> MTVGTLVASVLPATVFE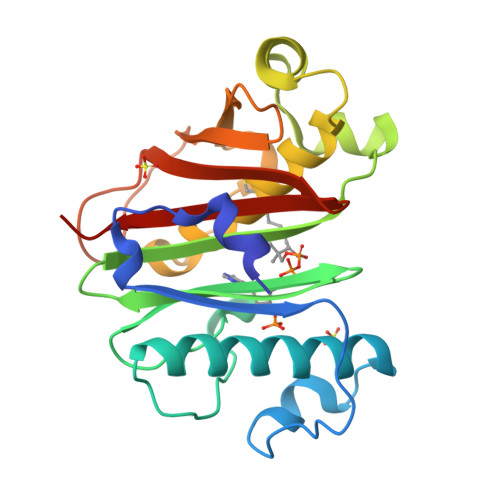DLAYAELYSDPPGLTPLPEEAPLIARSVAKRRNEFITVRHCARIALDQLGVPPAPILKGDKGEPCWPDGMVGSLTHCAGYRGAVVGRRDAVRSVGIDAEPHDVLPNGVLDAISLPAERADMPRTMPAALHWDRILFCAKEATYKAWFPLTKRWLGFEDAHITFETDSTGWTGRFVSRILIDGSTLSGPPLTTLRGRWSVERGLVLTAIVLLEHHHHHH>XDYLRELLKLELQAIKQYREALEYVKLPVLAKILEDE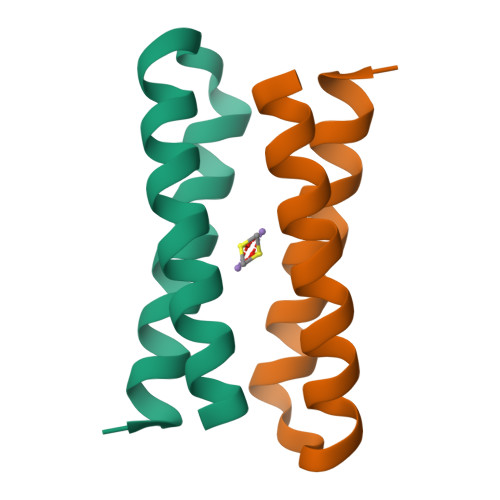EKHIEWLETILGX[3x]>AQSVPWGISRVQAPAAHNRGLTGSGVKVAVLDTGISTHPDLNIRGGASFVPGEPSTQDGNGHGTHVAGTIAALNNSIGVLGVAPSAELYAVKVLGASGSGSVSSIAQGLEWAGNNGMHVANLSLGSPSPSATLEQAVNSATSRGVLVVAASGNSGAGSISYPARYANAMAVGATDQNNNRASFSQYGAGLDIVAPGVNVQSTYPGSTYASLNGTSMATPHVAGAAALVKQKNPSWSNVQIRNHLKNTATSLGSTNLYGSGLVNAEAATR[2x];>[2x]ADPPPVHDTDGHELRADANY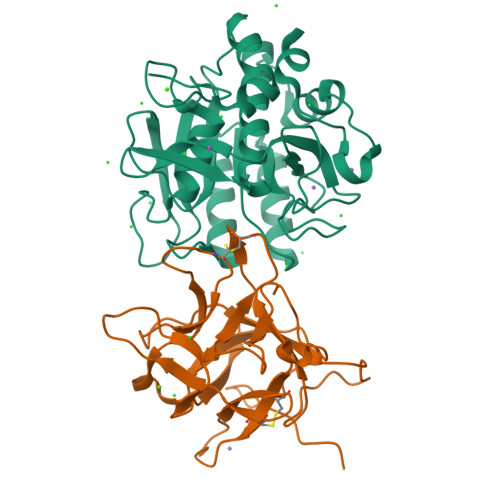YVLSANRAHGGGLTMAPGHGRHCPLFVSQDPNGQHDGFPVRITPYGVAPSDKIIRLSTDVRISFRAYTTCLQSTEWHIDSELAAGRRHVITGPVKDPSPSGRENAFRIEKYSGAEVHEYKLMSCGDWCQDLGVFRDLKGGAWFLGATEPYHVVVFKKAPPA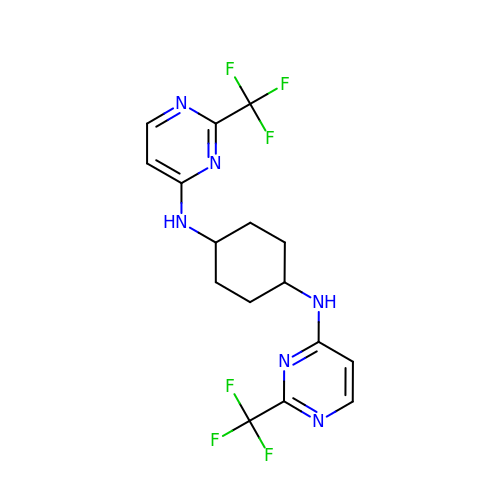~{N}1,~{N}4-bis[2-(trifluoromethyl)pyrimidin-4-yl]cyclohexane-1,4-diamine | C16 H16 F6 N6 | AWHJAHLJFNFTGF-AOOOYVTPSA-N>MDAQYDISFADVEKAHINIRDSIHLTPVLTSSILNQLTGRNLFFKCELFQKTGSFKIRGALNAVRSLVPDALERKPKAVVTHSSGNHGQALTYAAKLEGIPAYIVVPQTAPDCKKLAIQAYGASIVYCEPSDESRENVAKRVTEETEGIMVHPNQEPAVIAGQGTIALEVLNQVPLVDALVVPVGGGGMLAGIAITVKALKPSVKVYAAEPSNADDCYQSKLKGKLMPNLYPPETIADGVKSSIGLNTWPIIRDLVDDIFTVTEDEIKCATQLVWERMKLLIEPTAGVGVAAVLSQHFQTVSPEVKNICI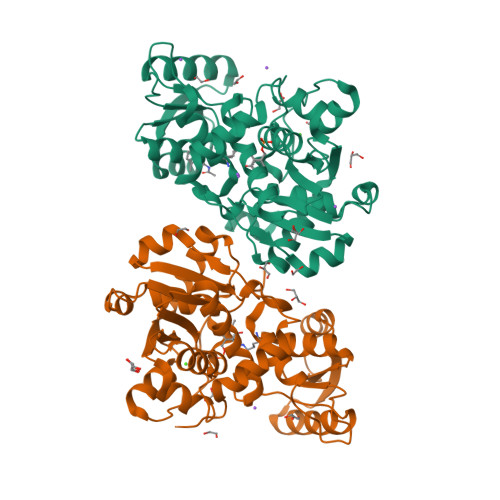VLSGGNVDLTSSITWVKQAERPASYQSVSVHHHHHH[4x]> ALSLPGSKSITARALFLAAAADGVTTLVRPLRSDDTEGFAEGLVRLGYRVGRTPDTWQVDGRPQGPAVAEADVYCRDGATTARFLPTLAAAGHGTYRFDASPQMRRRPLLPLSRALRDLGVDLRHEEAEGHHPLTVRAAGVEGGEVTLDAGQSSQYLTALL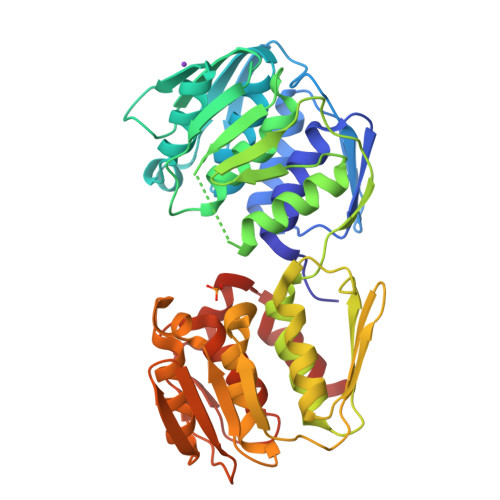LLGPLTRQGLRIRVTDLVSAPYVEITLAMMRAFGVEVAREGDVFVVPPGGYRATTYAIEPDASTASYFFAAAALTPGAEVTVPGLGTGALQGDLGFVDVLRRMGAEVSVGADATTVRGTGELRGLTANMRDISDTMPTLAAIAPFASAPVRIEDVANTRVKECDRLEACAENLRRLGVRVATGPDWIEIHPGPATGAQVTSYGDHRIVMSFAVTGLRVPGISFDDPGCVRKTFPGFHEAFAELRRGIGS>VECDFSPLLSGTPPQVYNFKRLVFTNCNYNLTKLLSLFSVNDFTCSQISPAAIASNCYSSLILDYFSYPLSMKSDLSVSSAGPISQFNYKQSFSNPTCLILATVPHNLTTITKPLKYSYINKCSRFLSDDRTEVPQLVNANQYSP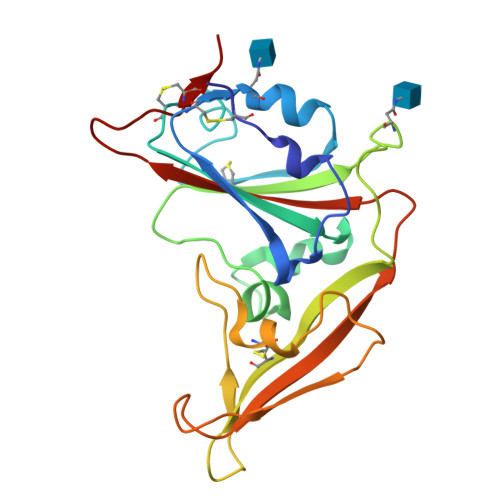CVSIVPSTVWEDGDYYRKQLSPLEGGGWLVASGSTVAMTEQLQMGFGITVQYGTDTNSVCPKL[2x]> GAFLDKPKMEKHNAQGQGNGLRYGLSSMQGWRVEMEAAHTAVIGLPSGLESWSFFAVYDGHAGSQVAKYCCEHLLDHITNNQDFKGSAGAPSVENVKNGIRTGFLEIDEHMRVMSEKKHGADRSGSTAVGVLISPQHTYFINCGDSRGLLCRNRKVHFFTQDHKPSNPLEKERIQNAGGSVMIQRVNGSLAVSRALGDFDYKCVHGKGPTEQLVSPEPEVHDIERSEEDDQFIILACDGIWDVMGNEELCDFVRSRLEVTDDLEKVCNEVVDTCLYKGSRDNMSVILICFPNAPKVSPEAVKKEAELDKYLECRVEEIIKKQGEGVPDLVHVMRTLASENIPSLPPGGELASKRNVIEAVYNRLNPY

The PP2Cα is the prototype PP2C family phosphatase for which the catalytic mechanisms and cellular functions have been well characterized. The active site of PP2C is located at a cleft between two central β sheets, and it harbors a binuclear metal ion site required for catalysis. In the crystal structure of PP2Cα, the M2 metal ion is directly coordinated to the primary chain carbonyl of the Gly61 and the side-chain carboxylate group of Asp60. In addition to these direct interactions, the M2 metal ion of PP2Cα also indirectly interacts with Glu37 and Asp38 through water-mediated hydrogen bonds.

We made a D38A mutation in PP2Cα, which eliminated the D38 side chain and abolished the indirect interaction between D38 and the M2 metal ion. To further elucidate the structural basis of the impaired function and catalysis of D38 mutants, we solved the crystal structures of PP2Cα-D38A and D38K with Mn2+ at 2.0 Å and 1.85 Å, respectively, and compared these structures with the PP2Cα-WT that was crystallized under similar conditions (1.95 Å). However, in contrast to the crystal structure of the PP2Cα-WT, the electron density for the M2 metal ion and the phosphate can't be clearly located in the D38A or D38K crystal structures. Specifically, one water (WAT11) between the D38 and D60 in the PP2Cα-WT crystal structure was replaced by two waters (WAT8 and WAT248) in the solvent channel between the A38 and D60 in the D38A crystal structure, which form specific H-bond with the main chain amide of G61. The positions of these two waters preclude M2 metal ion binding to the D38A mutant protein. Our crystal structures revealed that the D38A and D38K mutations altered the water-mediated hydrogen bond network and disrupted M2 metal ion binding with the maintenance of the protein folding and other active site conformations, which provide specific tools to investigate the functional role of the M2 metal ion among PP2C phosphatases. However, the overexpression of an equal amount of PP2Cα-D38A mutant as the wild type only slightly decreased the EGF-induced ERK phosphorylation, and the overexpression of the PP2Cα-D38K mutant has little effect on the ERK phosphorylation increase. Accordingly, the D38A decreased sulfate binding by 4-fold, and D38K decreased the sulfate binding by 10-fold. As a result, the βlg value of kcat decreased from −0.31 for PP2Cα-WT to −0.55 for D38A, and −0.44 for D38K. As a result, the βlg value for the kcat of H62N/D38A is −0.7, which is significantly lower than that of both H62N and D38A.>HGEKSQAAFMRMRTIHWYDLSWSKEKVKINETVEIKGKFHVFEGWPETVDEPDVAFLNVGMPGPVFIRKESYIGGQLVPRSVRLEIGKTYDFRVVLKARRPGDWHVHTMMNVQGGGPIIGPGKWITVEGSMSEFRNPVTTLTGQTVDLENYNEGNTYFWHAFWFAIGVAWIGYWSRRPIFIPRLLMVDAGRADELVSATDRKVAMGFLAATILIVVMAMSSANSKYPITIPLQAGTMRGMKPLELPAPTVSVKVEDATYRVPGRAMRMKLTITNHGNSPIRLGEFYTASVRFLDSDVYKDTTGYPEDLLAEDGLSVSDNSPLAPGETRTVDVTASDAAWEVYRLSDIIYDPDSRFAGLLFFFDATGNRQVVQIDAPLIPSFM[3x];>[3x]MSAAQSAVRSHAEAVQVSRTIDWMALFVVFFVIVGSYHIHAMLTMGDWDFWSDWKDRRLWVTVTPIVLVTFPAAVQSYLWERYRLPWGATVCVLGLLLGEWINRYFNFWGWTYFPINFVFPASLVPGAIILDTVLMLSGSYLFTAIVGAMGWGLIFYPGNWPIIAPLHVPVEYNGMLMSIADIQGYNYVRTGTPEYIRMVEKGTLRTFGKDVAPVSAFFSAFMSILIYFMWHFIGRWFSNERFLQST;>MHETKQGGEKRFTGAICRCSHRYNSMEVKMAATTIGGAAAAEAPLLDKKWLTFALAIYTVFYLWVRWYEGVYGWSA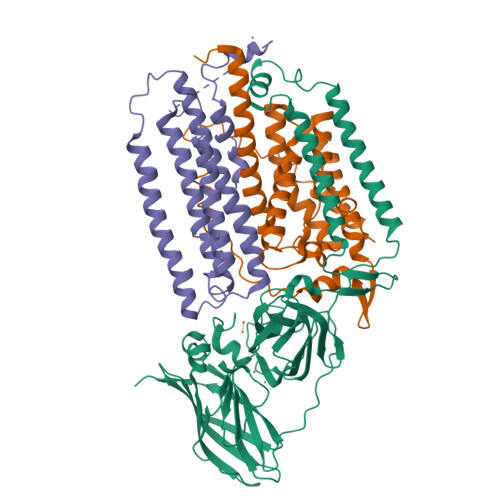GLDSFAPEFETYWMNFLYTEIVLEIVTASILWGYLWKTRDRNLAALTPREELRRNFTHLVWLVAYAWAIYWGASYFTEQDGTWHQTIVRDTDFTPSHIIEFYLSYPIYIITGFAAFIYAKTRLPFFAKGISLPYLVLVVGPFMILPNVGLNEWGHTFWFMEELFVAPLHYGFVIFGWLALAVMGTLTQTFYSFAQGGLGQSLCEAVDEGLIAK[3x]> MAFVATQGATVVDQTTLMKKYLQFVAALTDVNTPDETKLKMMQEVSENFENVTSSPQYSTFLEHIIPRFLTFLQDGEVQFLQEKPAQQLRKLVLEIIHRIPTNEHLRPHTKNVLSVMFRFLETENEENVLICLRIIIELHKQFRPPITQEIHHFLDFVKQIYKELPKVVNRYFENPQVIPENTVPPPEMVGMITTIAVKVNPEREDSETRTHSIIPRGSLSLKVLAELPIIVVLMYQLYKLNIHNVVAEFVPLIMNTIAIQVSAQARQHKLYNKELYADFIAAQIKTLSFLAYIIRIYQELVTKYSQQMVKGMLQLLSNCPAETAHLRKELLIAAKHILTTELRNQFIPCMDKLFDESILIGSGYTARETLRPLAYSTLADLVHHVRQHLPLSDLSLAVQLFAKNIDDESLPSSIQTMSCKLLLNLVDCIRSKSEQESGNGRDVLMRMLEVFVLKFHTIARYQLSAIFKKCKPQSELGAVEAALPGVPTAPAAPGPAPSPAPVPAPPPPPPPPPPATPVTPAPVPPFEKQGEKDKEDKQTFQVTDCRSLVKTLVCGVKTITWGITSCKAPGEAQFIPNKQLQPKETQIYIKLVKYAMQALDIYQVQIAGNGQTYIRVANCQTVRMKEEKEVLEHFAGVFTMMNPLTFKEIFQTTVPYMVERISKNYALQIVANSFLANPTTSALFATILVEYLLDRLPEMGSNVELSNLYLKLFKLVFGSVSLFAAENEQMLKPHLHKIVNSSMELAQTAKEPYNYFLLLRALFRSIGGGSHDLLYQEFLPLLPNLLQGLNMLQSGLHKQHMKDLFVELCLTVPVRLSSLLPYLPMLMDPLVSALNGSQTLVSQGLRTLELCVDNLQPDFLYDHIQPVRAELMQALWRTLRNPADSISHVAYRVLGKFGGSNRKMLKESQKLHYVVTEVQGPSITVEFSDCKASLQLPMEKAIETALDCLKSANTEPYYRRQAWEVIKCFLVAMMSLEDNKHALYQLLAHPNFTEKTIPNVIISHRYKAQDTPARKTFEQALTGAFMSAVIKDLRPSALPFVASLIRHYTMVAVAQQCGPFLLPCYQVGSQPSTAMFHSEENGSKGMDPLVLIDAIAICMAYEEKELCKIGEVALAVIFDVASIILGSKERACQLPLFSYIVERLCACCYEQAWYAKLGGVVSIKFLMERLPLTWVLQNQQTFLKALLFVMMDLTGEVSNGAVAMAKTTLEQLLMRCATPLKDEERAEEIVAAQEKSFHHVTHDLVREVTSPNSTVRKQAMHSLQVLAQVTGKSVTVIMEPHKEVLQDMVPPKKHLLRHQPANAQIGLMEGNTFCTTLQPRLFTMDLNVVEHKVFYTELLNLCEAEDSALTKLPCYKSLPSLVPLRIAALNALAACNYLPQSREKIIAALFKALNSTNSELQEAGEACMRKFLEGATIEVDQIHTHMRPLLMMLGDYRSLTLNVVNRLTSVTRLFPNSFNDKFCDQMMQHLRKWMEVVVITHKGGQRSDGNESISECGRCPLSPFCQFEEMKICSAIINLFHLIPAAPQTLVKPLLEVVMKTERAMLIEAGSPFREPLIKFLTRHPSQTVELFMMEATLNDPQWSRMFMSFLKHKDARPLRDVLAANPNRFITLLLPGGAQTAVRPGSPSTSTMRLDLQFQAIKIISIIVKNDDSWLASQHSLVSQLRRVWVSENFQERHRKENMAATNWKEPKLLAYCLLNYCKRNYGDIELLFQLLRAFTGRFLCNMTFLKEYMEEEIPKNYSIAQKRALFFRFVDFNDPNFGDELKAKVLQHILNPAFLYSFEKGEGEQLLGPPNPEGDNPESITSVFITKVLDPEKQADMLDSLRIYLLQYATLLVEHAPHHIHDNNKNRNSKLRRLMTFAWPCLLSKACVDPACKYSGHLLLAHIIAKFAIHKKIVLQVFHSLLKAHAMEARAIVRQAMAILTPAVPARMEDGHQMLTHWTRKIIVEEGHTVPQLVHILHLIVQHFKVYYPVRHHLVQHMVSAMQRLGFTPSVTIEQRRLAVDLSEVVIKWELQRIKDQQPDSDMDPNSSGEGVNSVSSSIKRGLSVDSAQEVKRFRTATGAISAVFGRSQSLPGADSLLAKPIDKQHTDTVVNFLIRVACQVNDNTNTAGSPGEVLSRRCVNLLKTALRPDMWPKSELKLQWFDKLLMTVEQPNQVNYGNICTGLEVLSFLLTVLQSPAILSSFKPLQRGIAACMTCGNTKVLRAVHSLLSRLMSIFPTEPSTSSVASKYEELECLYAAVGKVIYEGLTNYEKATNANPSQLFGTLMILKSACSNNPSYIDRLISVFMRSLQKMVREHLNPQAASGSTEATSGTSELVMLSLELVKTRLAVMSMEMRKNFIQAILTSLIEKSPDAKILRAVVKIVEEWVKNNSPMAANQTPTLREKSILLVKMMTYIEKRFPEDLELNAQFLDLVNYVYRDETLSGSELTAKLEPAFLSGLRCAQPLIRAKFFEVFDNSMKRRVYERLLYVTCSQNWEAMGNHFWIKQCIELLLAVCEKSTPIGTSCQGAMLPSITNVINLADSHDRAAFAMVTHVKQEPRERENSESKEEDVEIDIELAPGDQTSTPKTKELSEKDIGNQLHMLTNRHDKFLDTLREVKTGALLSAFVQLCHISTTLAEKTWVQLFPRLWKILSDRQQHALAGEISPFLCSGSHQVQRDCQPSALNCFVEAMSQCVPPIPIRPCVLKYLGKTHNLWFRSTLMLEHQAFEKGLSLQIKPKQTTEFYEQESITPPQQEILDSLAELYSLLQEEDMWAGLWQKRCKYSETATAIAYEQHGFFEQAQESYEKAMDKAKKEHERSNASPAIFPEYQLWEDHWIRCSKELNQWEALTEYGQSKGHINPYLVLECAWRVSNWTAMKEALVQVEVSCPKEMAWKVNMYRGYLAICHPEEQQLSFIERLVEMASSLAIREWRRLPHVVSHVHTPLLQAAQQIIELQEAAQINAGLQPTNLGRNNSLHDMKTVVKTWRNRLPIVSDDLSHWSSIFMWRQHHYQGKPTWSGMHSSSIVTAYENSSQHDPSSNNAMLGVHASASAIIQYGKIARKQGLVNVALDILSRIHTIPTVPIVDCFQKIRQQVKCYLQLAGVMGKNECMQGLEVIESTNLKYFTKEMTAEFYALKGMFLAQINKSEEANKAFSAAVQMHDVLVKAWAMWGDYLENIFVKERQLHLGVSAITCYLHACRHQNESKSRKYLAKVLWLLSFDDDKNTLADAVDKYCIGVPPIQWLAWIPQLLTCLVGSEGKLLLNLISQVGRVYPQAVYFPIRTLYLTLKIEQRERYKSDPGPIRATAPMWRCSRIMHMQRELHPTLLSSLEGIVDQMVWFRENWHEEVLRQLQQGLAKCYSVAFEKSGAVSDAKITPHTLNFVKKLVSTFGVGLENVSNVSTMFSSAASESLARRAQATAQDPVFQKLKGQFTTDFDFSVPGSMKLHNLISKLKKWIKILEAKTKQLPKFFLIEEKCRFLSNFSAQTAEVEIPGEFLMPKPTHYYIKIARFMPRVEIVQKHNTAARRLYIRGHNGKIYPYLVMNDACLTESRREERVLQLLRLLNPCLEKRKETTKRHLFFTVPRVVAVSPQMRLVEDNPSSLSLVEIYKQRCAKKGIEHDNPISRYYDRLATVQARGTQASHQVLRDILKEVQSNMVPRSMLKEWALHTFPNATDYWTFRKMFTIQLALIGFAEFVLHLNRLNPEMLQIAQDTGKLNVAYFRFDINDATGDLDANRPVPFRLTPNISEFLTTIGVSGPLTASMIAVARCFAQPNFKVDGILKTVLRDEIIAWHKKTQEDTSSPLSAAGQPENMDSQQLVSLVQKAVTAIMTRLHNLAQFEGGESKVNTLVAAANSLDNLCRMDPAWHPWL;> MHHGTGPQNVQHQLQRSRACPGSEGEEQPAHPNPPPSPAAPFAPSASPSAPQSPSYQIQQLMNRSPATGQNVNITLQSVGPVVGGNQQITLAPLPLPSPTSPGFQFSAQPRRFEHGSPSYIQVTSPLSQQVQTQSPTQPSPGPGQALQNVRAGAPGPGLGLCSSSPTGGFVDASVLVRQISLSPSSGGHFVFQDGSGLTQIAQGAQVQLQHPGTPITVRERRPSQPHTQSGGTIHHLGPQSPAAAGGAGLQPLASPSHITTANLPPQISSIIQGQLVQQQQVLQGPPLPRPLGFERTPGVLLPGAGGAAGFGMTSPPPPTSPSRTAVPPGLSSLPLTSVGNTGMKKVPKKLEEIPPASPEMAQMRKQCLDYHYQEMQALKEVFKEYLIELFFLQHFQGNMMDFLAFKKKHYAPLQAYLRQNDLDIEEEEEEEEEEEEKSEVINDEVKVVTGKDGQTGTPVAIATQLPPKVSAAFSSQQQPFQQALAGSLVAGAGSTVETDLFKRQQAMPSTGMAEQSKRPRLEVGHQGVVFQHPGADAGVPLQQLMPTAQGGMPPTPQAAQLAGQRQSQQQYDPSTGPPVQNAASLHTPLPQLPGRLPPAGVPTAALSSALQFAQQPQVVEAQTQLQIPVKTQQPNVPIPAPPSSQLPIPPSQPAQLALHVPTPGKVQVQASQLSSLPQMVASTRLPVDPAPPCPRPLPTSSTSSLAPVSGSGPGPSPARSSPVNRPSSATNKALSPVTSRTPGVVASAPTKPQSPAQNATSSQDSSQDTLTEQITLENQVHQRIAELRKAGLWSQRRLPKLQEAPRPKSHWDYLLEEMQWMATDFAQERRWKVAAAKKLVRTVVRHHEEKQLREERGKKEEQSRLRRIAASTAREIECFWSNIEQVVEIKLRVELEEKRKKALNLQKVSRRGKELRPKGFDALQESSLDSGMSGRKRKASISLTDDEVDDEEETIEEEEANEGVVDHQTELSNLAKEAELPLLDLMKLYEGAFLPSSQWPRPKPDGEDTSGEEDADDCPGDRESRKDLVLIDSLFIMDQFKAAERMNIGKPNAKDIADVTAVAEAILPKGSARVTTSVKFNAPSLLYGALRDYQKIGLDWLAKLYRKNLNGILADEAGLGKTVQIIAFFAHLACNEGNWGPHLVVVRSCNILKWELELKRWCPGLKILSYIGSHRELKAKRQEWAEPNSFHVCITSYTQFFRGLTAFTRVRWKCLVIDEMQRVKGMTERHWEAVFTLQSQQRLLLIDSPLHNTFLELWTMVHFLVPGISRPYLSSPLRAPSEESQDYYHKVVIRLHRVTQPFILRRTKRDVEKQLTKKYEHVLKCRLSNRQKALYEDVILQPGTQEALKSGHFVNVLSILVRLQRICNHPGLVEPRHPGSSYVAGPLEYPSASLILKALERDFWKEADLSMFDLIGLENKITRHEAELLSKKKIPRKLMEEISTSAAPAARPAAAKLKASRLFQPVQYGQKPEGRTVAFPSTHPPRTAAPTTASAAPQGPLRGRPPIATFSANPEAKAAAAPFQTSQASASAPRHQPASASSTAASPAHPAKLRAQTTAQASTPGQPPPQPQAPSHAAGQSALPQRLVLPSQAQARLPSGEVVKIAQLASITGPQSRVAQPETPVTLQFQGSKFTLSHSQLRQLTAGQPLQLQGSVLQIVSAPGQPYLRAPGPVVMQTVSQAGAVHGALGSKPPAGGPSPAPLTPQVGVPGRVAVNALAVGEPGTASKPASPIGGPTQEEKTRLLKERLDQIYLVNERRCSQAPVYGRDLLRICALPSHGRVQWRGSLDGRRGKEAGPAHSYTSSSESPSELMLTLCRCGESLQDVIDRVAFVIPPVVAAPPSLRVPRPPPLYSHRMRILRQGLREHAAPYFQQLRQTTAPRLLQFPELRLVQFDSGKLEALAILLQKLKSEGRRVLILSQMILMLDILEMFLNFHYLTYVRIDENASSEQRQELMRSFNRDRRIFCAILSTHSRTTGINLVEADTVVFYDNDLNPVMDAKAQEWCDRIGRCKDIHIYRLVSGNSIEEKLLKNGTKDLIREVAAQGNDYSMAFLTQRTIQELFEVYSPMDDAGFPVKAEEFVVLSQEPSVTETIAPKIARPFIEALKSIEYLEEDAQKSAQEGVLGPHTDALSSDSENMPCDEEPSQLEELADFMEQLTPIEKYALNYLELFHTSIEQEKERNSEDAVMTAVRAWEFWNLKTLQEREARLRLEQEEAELLTYTREDAYSMEYVYEDVDGQTEVMPLWTPPTPPQDDSDIYLDSVMCLMYEATPIPEAKLPPVYVRKERKRHKTDPSAAGRKKKQRHGEAVVPPRSLFDRATPGLLKIRREGKEQKKNILLKQQVPFAKPLPTFAKPTAEPGQDNPEWLISEDWALLQAVKQLLELPLNLTIVSPAHTPNWDLVSDVVNSCSRIYRSSKQCRNRYENVIIPREEGKSKNNRPLRTSQIYAQDENATHTQLYTSHFDLMKMTAGKRSPPIKPLLGMNPFQKNPKHASVLAESGINYDKPLPPIQVASLRAERIAKEKKALADQQKAQQPAVAQPPPPQPQPPPPPQQPPPPLPQPQAAGSQPPAGPPAVQPQPQPQPQTQPQPVQAPAKAQPAITTGGSAAVLAGTIKTSVTGTSMPTGAVSGNVIVNTIAGVPAATFQSINKRLASPVAPGALTTPGGSAPAQVVHTQPPPRAVGSPATATPDLVSMATTQGVRAVTSVTASAVVTTNLTPVQTPARSLVPQVSQATGVQLPGKTITPAHFQLLRQQQQQQQQQQQQQQQQQQQQQQQQQQQQQTTTTSQVQVPQIQGQAQSPAQIKAVGKLTPEHLIKMQKQKLQMPPQPPPPQAQSAPPQPTAQVQVQTSQPPQQQSPQLTTVTAPRPGALLTGTTVANLQVARLTRVPTSQLQAQGQMQTQAPQPAQVALAKPPVVSVPAAVVSSPGVTTLPMNVAGISVAIGQPQKAAGQTVVAQPVHMQQLLKLKQQAVQQQKAIQPQAAQGPAAVQQKITAQQITTPGAQQKVAYAAQPALKTQFLTTPISQAQKLAGAQQVQTQIQVAKLPQVVQQQTPVASIQQVASASQQASPQTVALTQATAAGQQVQMIPAVTATAQVVQQKLIQQQVVTTASAPLQTPGAPNPAQVPASSDSPSQQPKLQMRVPAVRLKTPTKPPCQ

The human Tat-interactive protein, 60 kDa (TIP60) complex, a fusion of the yeast nucleosome acetyltransferase of histone H4 (NuA4) and switch/sucrose nonfermentable related 1 (SWR1) complexes, is involved in both histone acetylation and H2A.Z-H2B histone exchange and is essential for cell viability, playing a role, among other cellular processes, in gene regulation and DNA double-strand break repair. TIP60 can modify nucleosomes through covalent and noncovalent mechanisms by using its histone acetyltransferase (HAT) module and its E1A binding protein P400 (EP400) chromatin remodeler subunit, respectively. TIP60 consists of five modules, including TINTIN, HAT, TRRAP, ARP, and BASE, each with distinct functions. Within the complex, the EP400 protein functions as a major scaffold, making interactions with all the functional and structural modules, a role similar to that of the Eaf1 subunit in the yeast NuA4 complex and of the Swr1 subunit in the SWR1 complex, the two subunits of which EP400 is a merge.

Only 137 amino acids of EP400 were resolved in our structure in addition to TRRAP itself. This fragment of EP400 corresponds to the SANT and HD domains, which interact with the focal adhesion targeting (FAT) and Huntington, elongation factor 3, PR65/A, TOR (HEAT) domains of TRRAP. Within the triangle-shaped SANT domain, residues H2397, R2413, H2464, and K2469 anchor two ends of the triangle to two acidic patches within the FAT and HEAT domains, whereas D2406, in the middle of the SANT domain, interacts with a positively charged patch of TRRAP. Of particular interest, H2397L and R2413Q have been identified as cancer-associated mutations. Following the SANT domain, the HD domain of EP400 interacts with the phosphatidylinositol-3 kinase-related kinase (PIKK)–like domain of TRRAP through hydrophobic interactions involving residues L2498, I2503, Y2505, L2509, P2511, and I2512. The robust interactions of the SANT and HD domains with TRRAP tether it securely to the rest of the TIP60 complex. By contrast, a long flexible linker of EP400 connects TRRAP to the rest of TIP60, allowing a far reach of the acetylation and histone exchange functionalities from the site of recruitment. Of notice, the SANT and HD domains, which follow the EP400 linker, occupy the footprint of the structural component SUPT20H on the surface of the TRRAP subunit of the human SAGA complex, thereby preventing the formation of a hybrid complex.>[8x]MTMASVPASRYLTDMTLEEMSRDWSMLIPKQKVAGPLCIRMDQAIMDKNIILKANFSVIFDRLETLILLRAFTEEGAIVGEISPLPSLPGHTAEDVKNAVGVLIGGLEWNDNTVRVSETLQRFAWRSSNENGRPPLTPKQKREMAGTIRSEV

During infection the influenza A virus NS1 protein participates in multiple protein-RNA and protein-protein interactions to perform a plethora of functions. The N-terminal 73 amino-acid residues of NS1 form a symmetrical homodimeric RNA-binding domain (RBD), which is connected to the central effector domain (ED; residues 86-204) via an inter-domain linker. Present models of the tertiary and quaternary structures of NS1 indicate that the protein possesses two globular domains, each capable of forming independent homodimeric interactions. Our bioinformatic analyses indicate that the N-terminal RBD forms a very stable homodimer, while the predominant and ubiquitous helix-helix contacts between C-terminal EDs bear many similarities with weak transient interfaces.

In contrast, several possible ED homodimer interfaces have been proposed based upon crystal structures obtained using NS1 proteins from various strains. While the helix-helix interface appears to be the only dimeric form of NS1 ED consistently observed in all crystal structures, it remains possible that other dimeric states (such as the strand-strand dimer) contribute to dimerization in solution. Although the helix-helix dimer interface is shared by all structures of the NS1 ED, and may have some biological role in that RNA-binding activity of NS1 is affected by its disruption, we noted that in all helix-helix structures the arrangement of the two ED monomers differs markedly relative to one another. However, at this same concentration we routinely observe complete dimerization of the PR8 and Alb/76 NS1 EDs. A key aspect of our functional model is the instability and flexibility of the NS1 ED helix-helix dimer, which seems weak and transient in vitro, but may be slightly more stable in the context of the full-length protein, or become more permanent in the presence of certain binding partners. ED dimer flexibility is likely permitted by the presence of several glycine residues at the homodimer interface (a putative GxxxG protein-protein interaction motif) that allow the two helices to rotate easily relative to one another.(3~{S},7~{R},10~{R},11~{R},13~{S})-4-[(3~{S},6~{R},8~{a}~{S})-1'-[(2~{S})-2-acetamido-3-(2-chlorophenyl)propanoyl]-5-oxidanylidene-spiro[1,2,3,8~{a}-tetrahydroindolizine-6,2'-pyrrolidine]-3-yl]carbonyl-11-methyl-2-oxidanylidene-1,4-diazatricyclo[8.3.0.0^{3,7}]tridec-8-ene-13-carboxylic 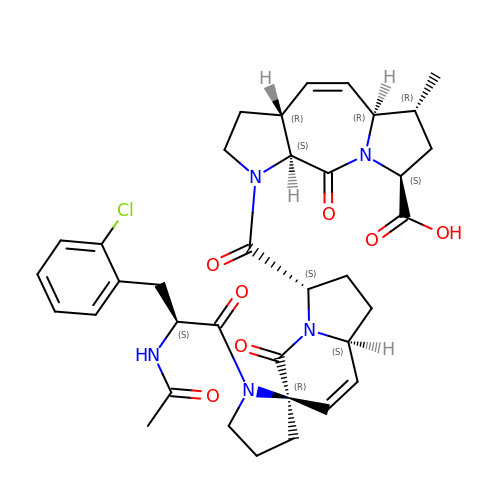acid | C36 H42 Cl N5 O7 | FZILKQWAXMUHKU-PKMCVEQOSA-N>[3x]MNAWD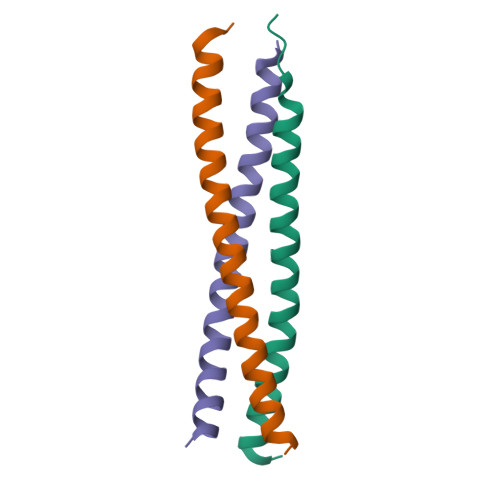RTLIENGEKITSLHREVEKVKLDQKRLDQELDFILSQQKELEDLLSP>[2x]GSHNDKDLSTWQTFRRLWPTIAPFKAGLIVAGVALILNAASDTFMLSLLKPLLDDGFGKTDRSVLVWMPLVVIGLMILRGITSYVSSYCISWVSGKVVMTMRRRLFGHMMGMPVSFFDKQSTGTLLSRITYDSEQVASSSSGALITVVREGASIIGLFIMMFYYSWQLSIILIVLAPIVSIAIRVVSKRFRNISKNMQNTMGQVTTSAEQMLKGHKEVLIFGGQEVETKRFDKVSNRMRLQGMKMVSASSISDPIIQLIASLALAFVLYAASFPSVMDSLTAGTITVVFSSMIALMRPLKSLTNVNAQFQRGMAACQTLFTILDSEQEKDEGKRVIERATGDVE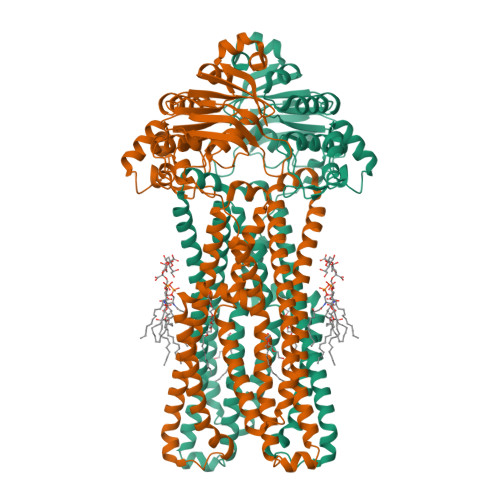FRNVTFTYPGRDVPALRNINLKIPAGKTVALVGRSGSGKSTIASLITRFYDIDEGEILMDGHDLREYTLASLRNQVALVSQNVHLFNDTVANNIAYARTEQYSREQIEEAARMAYAMDFINKMDNGLDTVIGENGVLLSGGQRQRIAIARALLRDSPILILDEATSALDTESERAIQAALDELQKNRTSLVIAHRLSTIEKADEIVVVEDGVIVERGTHNDLLEHRGVYAQLHKMQFGQ> MATNKERLFAAGALGPGSGYPGAGFPFAFPGALRGSPPFEMLSPSFRGLGQPDLPKEMASLSVETQSTSSEEMVPSSPSPPPPPRVYKPCFVCNDKSSGYHYGVSSCEGCKGFFRRSIQKNMVYTCHRDKNCIINKVTRNRCQYCRLQKCFEVGMSKEAVRNDRNKKKKEVKEEGSPDSYELSPQLEELITKVSKAHQETFPSLCQLGKYTTNSSADHRVQLDLGLWDKFSELATKCIIKIVEFAKRLPGFTGLSIADQITLLKAACLDILMLRICTRYTPEQDTMTFSDGLTLNRTQMHNAGFGPLTDLVFAFAGQLLPLEMDDTETGLLSAICLICGDRMDLEEPEKVDKLQEPLLEALRLYARRRRPSQPYMFPRMLMKITDLRGISTKGAERAITLKMEIPGPMPPLIREMLENPEMFEDDSSQPGPHPNASSEDEVPG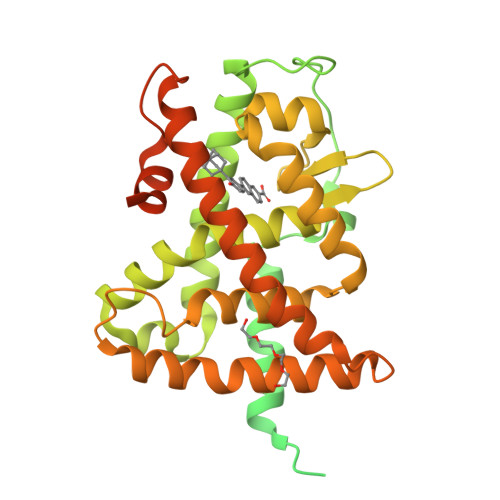GQGKGGLKSPA> MGSHHHHHHENLYFQGSIKFRVIFK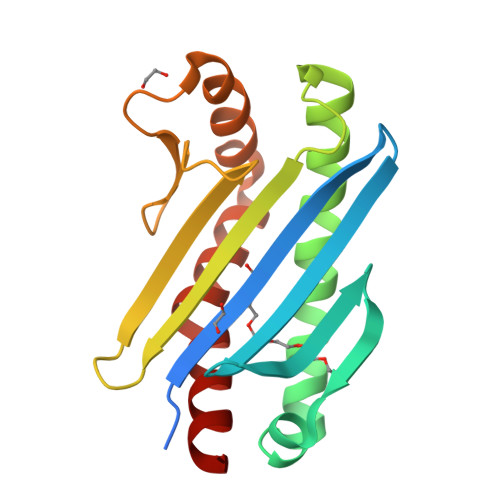VTVLSEDEVEVVFEVYLGDELVVKLVNFVTEYVAPAWTRAVPPEVAEALRKAVIEWGKGVAELFKKFVKKYGIPYGSVFEIVIGYDAATDTSFNEILVDGKPVISFDGEKFVVNEGAPKEFEPVVEELNANKELIEGLKFFLNVLGPLAARRLAAAA> MAEIVLDHVNKSYPDGHTAVRDLNLTIADGEFLILVGPSGCGKTTTLNMIAGLEDISSGELRIAGERVNEKAPKDRDIAMVFQSYALYPHMTVRQNIAFPLTLAKMRKADIAQKVSETAKILDLTNLLDRKPSQLSGGQRQRVAMGRAIVRHPKAFLMDEPLSNLDAKLRVQMRGEIAQLQRRLGTTTVYVTHDQTEAMTLGDRVVVMYGGIAQQIGTPEELYERPANLFVAGFIGSPAMNF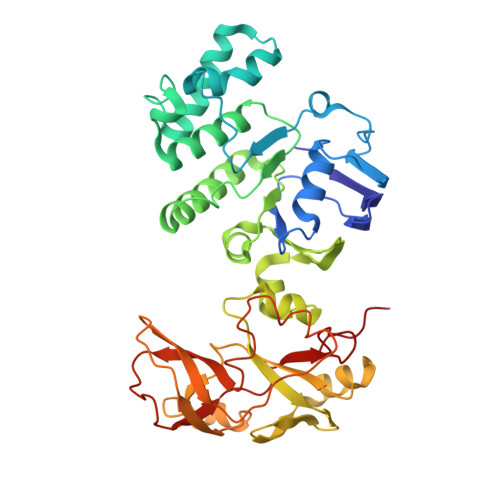FPARLTAIGLTLPFGEVTLAPEVQGVIAAHPKPENVIVGVRPEHIQDAALIDAYQRIRALTFQVKVNLVESLGADKYLYFTTESPAVHSVQLDELAEVEGESALHENQFVARVPAESKVAIGQSVELAFDTARLAVFDADSGANLTIPHRA> MNGIHDVGGMDGFGKVMYVKEEEDIYFTHDWERLAFGLVAGCMAQGLGMKAFD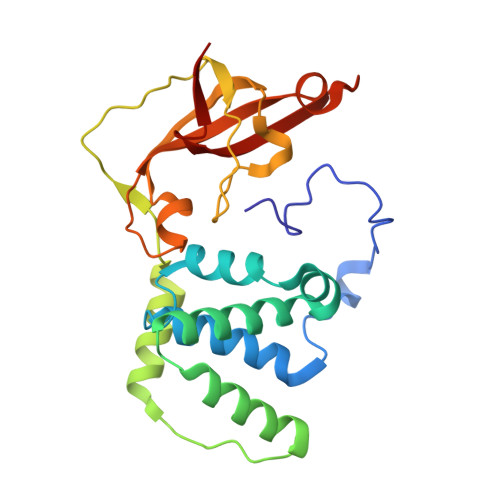EFRIGIELMRPVDYLTSSYYGHWIATVAYNLVDTGVLDEKELEERTEVFLKKPDTKIPRREDPALVKLVEKALYDGLSPLREISASPRFKVGERIKTKNIHPTGHTRFPRYARVKYGVIDEVYGAHVFPDDAAHRKGENPQYLYRVRFEAEELWGYKQKDSVYIDLWESYMEPVSH> GGDRVKKLINSQISLLIGKGLHEFDSLRDPEVNDFRTKMRQFCEEAAAHRQQLGWVEWLQYSFPLQLEPSARGWRAGLLRVSNRALLVNVKFEGSEESFTFQVSTKDMPLALMACALRKKATVFRQPLVEQPEEYALQVNGRHEYLYGNYPLCHFQYICSCLHSGLTPHLTMVHSSSILAMRDEQSNPAPQVQKPRAKPPPIPAKKPSSVSLWSLEQPFSIELIEGRKVNADERMKLVVQAGLFHGNEMLCKTVSSSEVNVCSEPVWKQRLEFDISVCDLPRMARLCFALYAVVEKAKKARSTKKKSKKADCPIAWANLMLFDYKDQLKTGERCLYMWPSVPDEKGELLNPAGTVRGNPNTESAAALVIYLPEVAPHPVYFPALEKILELGRHGERGRITEEEQLQLREILERRGSGELYEHEKDLVWKMRHEVQEHFPEALARLLLVTKWNKHEDVAQMLYLLCSWPELPVLSALELLDFSFPDCYVGSFAIKSLRKLTDDELFQYLLQLVQV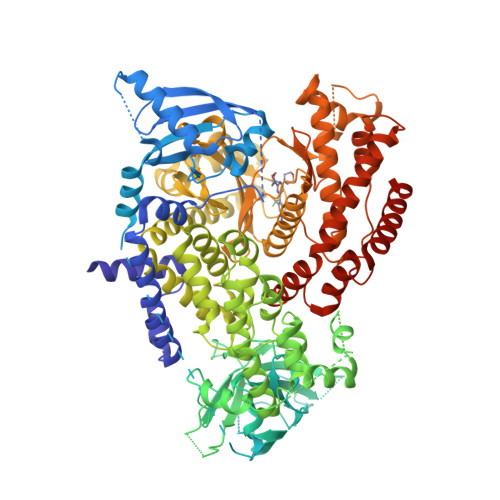LKYESYLDCELTKFLLGRALANRKIGHFLFWHLRSEMHVPSVALRFGLIMEAYCRGSTHHMKVLMKQGEALSKLKALNDFVKVSSQKTTKPQTKEMMHMCMRQETYMEALSHLQSPLDPSTLLEEVCVEQCTFMDSKMKPLWIMYSSEEAGSAGNVGIIFKNGDDLRQDMLTLQMIQLMDVLWKQEGLDLRMTPYGCLPTGDRTGLIEVVLHSDTIANIQLNKSNMAATAAFNKDALLNWLKSKNPGEALDRAIEEFTLSCAGYCVATYVLGIGDRHSDNIMIRESGQLFHIDFGHFLGNFKTKFGINRERVPFILTYDFVHVIQQGKTNNSEKFERFRGYCERAYTILRRHGLLFLHLFALMRAAGLPELSCSKDIQYLKDSLALGKTEEEALKHFRVKFNEALRESWKTKVNWLAHNVSKDNRQ> MRGSHHHHHHGSRVMVIGGDGYCGWATALHLSKKNYEVCIVDNLVRRLFDHQLGLESLTPIASIHDRISRWKALTGKSIELYVGDICDFEFLAESFKSFEPDSVVHFGEQRSAPYSMIDRSRAVYTQHNNVIGTLNVLFAIKEFGEECHLVKLGAMGEYGTPNIDIEEGYITITHNGRTDTLPYPKQASSFYHLSKVHDSHNIAFTCKAWGIRATDLNQGVVYGVKTDETEMHEELRNRLDYDAVFGTALNRFCVQAAVGHPLTVYGKGGQTRGYLDIRDTVQCVEIAIANPAKAGEFRVFNQFTEQFSVNE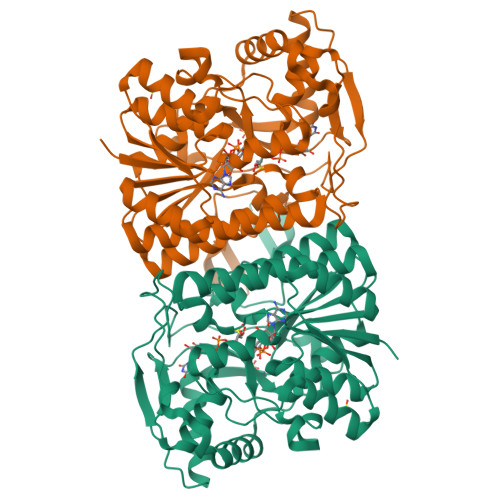LASLVTKAGSKLGLDVKKMTVPNPRVEAEEHYYNAKHTKLMELGLEPHYLSDSLLDSLLNFAVQFKDRVDTKQIMPSVSWKKIGVKTKSMTT> MATAQSNSPRVFCIGTADTKFDELRFLSEHVRSSLNSFSNKSSFKVGVTVVDVSTSWKETNSCADFDFVPSKDVLSCHTLGEETMGTFADTRGLAIAIMSKALETFLSIANDEQNLAGVIGLGGSGGTSLLSSAFRSLPIGIPKVIISTVASGQTESYIGTSDLVLFPSVVDICGINNVSKVVLSNAGAAFAGMVIGRLESSKEHSITNGKFTVGVTMFGVTTPCVNAVKERLVKEGYETLVFHATGVGGRAMEDLVRGGFIQGVLDITTTEVADYVVGGVMACDSSRFDAILEKKIPLVLSVGALDMVNFGPKTTIPPEFQQRKIHEHNEQVSLMRTTVGENKKFAAFIAEKLNKASSSVCVCLPEKGVSALDAPGKDFYDPEATSCLTRELQMLLENNERC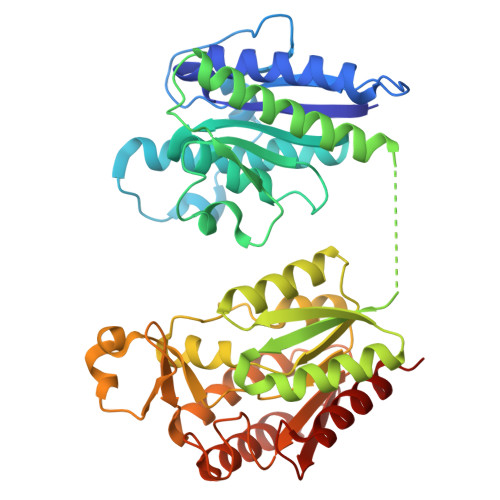QVKVLPYHINDAEFANALVDSFLEISPK> PYVEIIEQPKQRGMRFRYKCEGRSAGSIPGERSTDTTKTHPTIKINGYTGPGTVRISLVTKDPPHRPHPHELVGKDCRDGYYEADLCPDRSIHSFQNLGIQCVKKRDLEQAISQRIQTNNNPFHVPIEEQRGDYDLNAVRLCFQVTVRDPAGRPLLLTPVLSHPIFDNRAPNTAELKICRVNRNSGSCLGGDEIFLLCDKVQKEDIEVYFTGPGWEARGSFSQADVHRQVAIVFRTPPYADPSLQAPVRVSMQLRRPSDRELSEPMEFQYLPDTDDRHRIEEKRKR;> ASNLKIVRMDRTAGCVTGGEEIYLLCDKVQKDDIQIRFYEEEENGGVWEGFGDFSPTDVHRQFAIVFKTPKY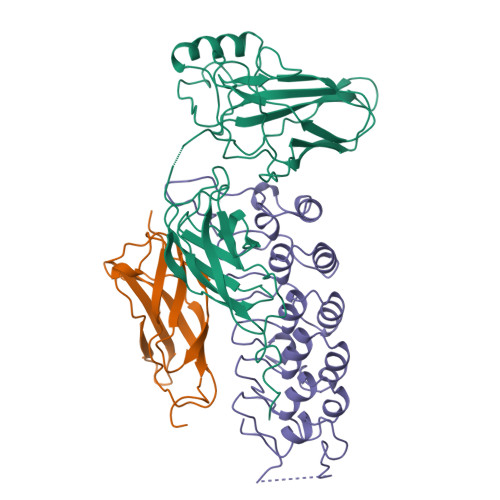KDVNITKPASVFVQLRRKSDLETSEPKPFLYYPEIKDKEEVQRKRQK;> KQQLTEDGDSFLHLAIIHEEKALTMEVIRQVKGDLAFLNFQNNLQQTPLHLAVITNQPEIAEALLGAGCDPELRDFRGNTPLHLACEQGCLASVGVLTQSCTTPHLHSILKATNYNGHTCLHLASIHGYLGIVELLVSLGADVNAQEPCNGRTALHLAVDLQNPDLVSLLLKCGADVNRVTYQGYSPYQLTWGRPSTRIQQQLGQLTLENLQMLPESEDEESYDTESEFTEFTEDE(3S,4S,5R)-3-(3-bromo-4-hydroxybenzyl)-5-[(3-cyclopropylbenzyl)amino]tetrahydro-2H-thiopyran-4-ol 1,1-dioxide | C22 H26 Br N 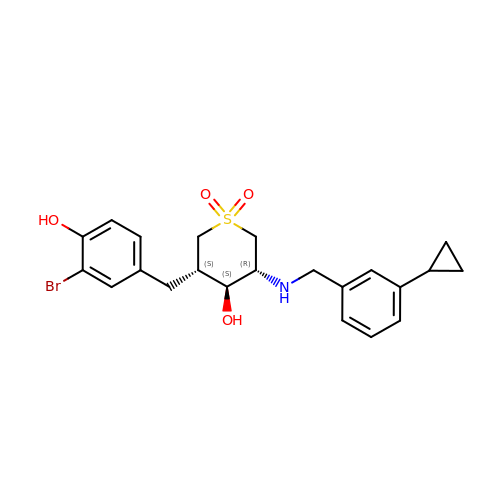O4 S | NDEIDRFQAYLHLT-CBQOVEMMSA-N> MGHNNTKGNRKFIKGRYTANAAKGERLVSSEFLLTFAGHEDISVLVRTSQIPEMTREDVEDYGPNGVKFNQHGPIR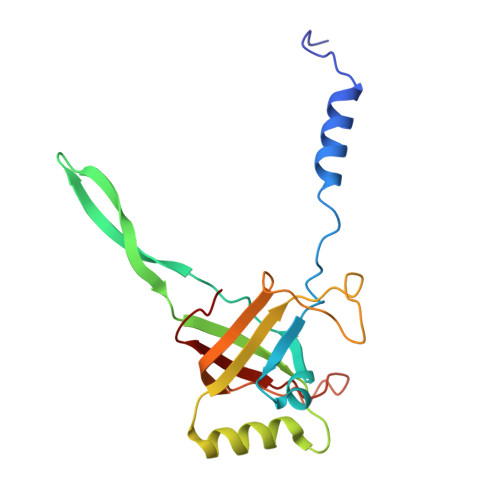NSGEIQVQCVETIEGDILQFIKDRIAAKDYVDITMAATPESKSSGVNAVTKAATTIEMLDCKIYSDAIDFSTEDVTAAVRPSLRIVYNWIEWD>[2x]SNIPYTQLDMAVVQNRPAGSLRRFVVLVVGETTRAANWGLNGYSRQTTPLLAARGDEIVNFPQVRSCGTSTAHSLPCMFSTFDRTDYDEIKAEHQDNLLDIVQRAGVEVTWLENDSGCKGVCGKVPNTDVTSLNLPEYCRNGECLDNILLTKFDEVLNKNDKDAVLILH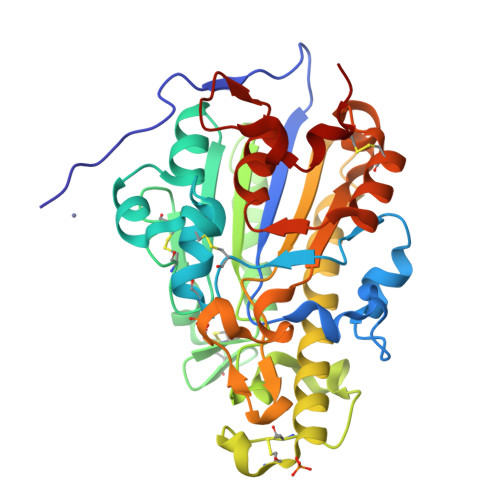TIGSHGPTYYERYTEAERKFTPTCDTNEINKCTRATLVNTYDNTVLYVDQFIDKVIRKLENRDDLESVVHYVSDHGESLGENGMYLHAAPYAIAPSGQTHIPMVMWFSKAFRQHGGIDFQCLKQKAAENEYSHDHYFSTVLGLMDISNSQTYRKEMDILAACRRPR> MSSLQKRPGPGNSSQPTERPRKESILDLSRYQ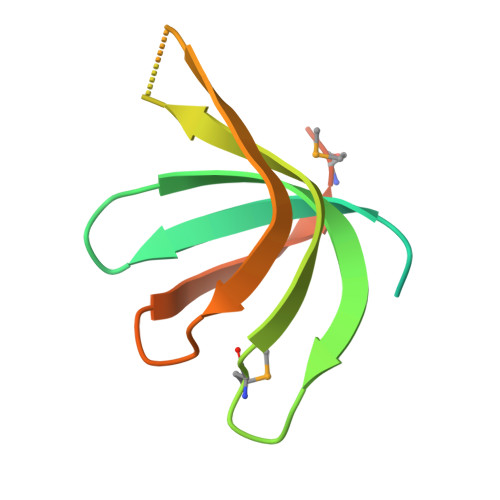DQRIQATFTGGRQITGILKGFDQLMNLVLDDVEEQLRNPEDGKLTGAIRKLGLVVVRGTTLVLIAPMDGSEEIPNPFVQAE>MALADGAAAPVAVTSYAQQPLKLVQEKASDGDGSAELELGLRYVFGSDGVKNVPLGVSWINKAALKGIPQAEHEMGSLYLMGIGVAQSNVMAVAWYRKAAIQGYAPSQTAMGYAYEEGAGVPQDADLA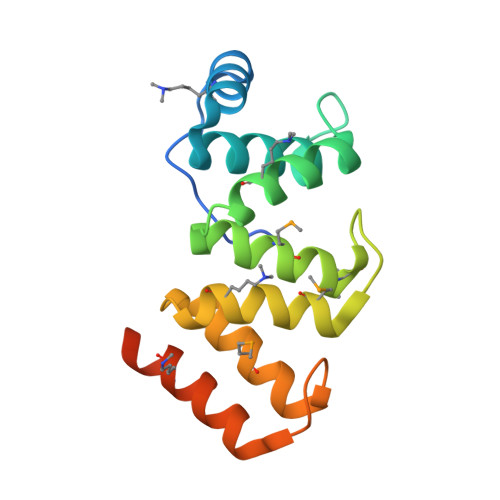RYWFDKAAAQGNGIAVESLEGGM[4x]>SLGSDADSAGSLI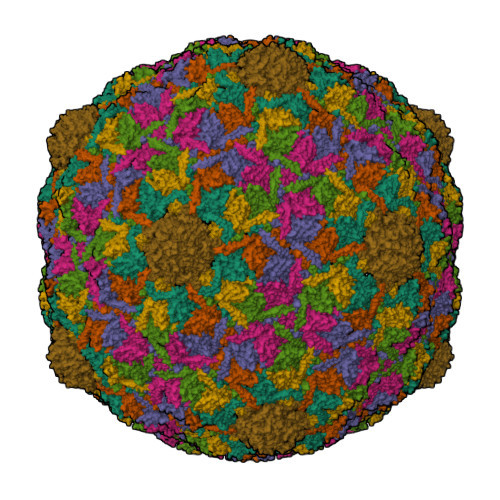QPMQIPGIIMPGLRRLTIRDLLAQGRTSSNALEYVREEVFTNNADVVAEKALYPESDITFSKQTANVKTIAHWVQASRQVMDDAPMLQSYINNRLMYGLALKEEGQLLNGDGTGDNLEGLNKVATAYDTSLNATGDTRADIIAHAIYQVTESEFSASGIVLNPRDWHNIALLKDNEGRYIFGGPQAFTSNIMWGLPVVPTKAQAAGTFTVGGFDMASQVWDRMDATVEVSREDRDNFVKNMLTILCEERLALAHYRPTAIIKGTFSSGS[7x]> AKYTGKCTKSKNECKYKNDAGKDTFIKCPKFDNKKCTKDNNKCTVDTYNNAVDCD

PAF is a small (∼6.2 kDa, 55 residues) lysine-rich protein (13 × Lys, pI ≃ 9) and a potent agent against Aspergillus species and dermatophytes. The NMR structure is a twisted β-barrel composed of five antiparallel β-strands and stabilized by three disulfide bridges. Lys30, Phe31, Lys34, Lys35 and Lys38 (loop 3) belong to a conserved region of PAF that is important for antifungal activity. Despite the varying size and conformational flexibility, sclx4, sclx6 and sclx8 bound similarly the Pro29-Lys30-Phe31 motif in loop 3.

In contrast, PAF–sclx4 mixtures were crystallized readily from solutions containing PEG and sodium acetate. Sclx4, locked in the cone conformation, encapsulates the side chain of a single lysine (Lys30), as observed previously in different protein-clx4 complexes. Depending on the ligand size/conformation, the noncovalent contacts varied in their type and multiplicity. The PAF–sclx4 complex [Fig. 2(a)] was similar to cytochrome c–sclx4, involving a salt bridge and CH—π/cation—π bonds with the encapsulated lysine. Hydrogen bonds to the backbone amide NHs of Lys30, Phe31 and Asp32 were evident and the aromatic ring of Phe31 was in van der Waals contact with an sclx4 methylene bridge. Considering symmetry mates [Fig. 4(a)], sclx4 formed substantial interfaces (>150 Å2) with three proteins. Interestingly, a salt bridge was formed with the Nα of Ala1. Salt bridges also occurred with Lys2, Lys17, Lys22 and Lys35, emphasizing a substantial charge–charge component to complexation. In total, the protein–sclx4 interfaces buried ∼660 Å2 of protein. In the crystal structure, all of these residues occurred in the vicinity of sclx4.> MPPKQTKVVASRKTVMPISRAGRAQIRRKDSNTQNNMNDQGMEDEEIDQQREGMKNQYEQLTAQELNEDMPSKMLEPKNPQAPKNITVYDYYTRKFKTDELVDQMIVHFSMDGDYIWKESNEYKTQEEIRDTKKALIKEAMRKQESEEPGANHDEEAIKQTLRNKFNYNTRECQTINPSIRERGVSTEPPPSDTICGNITQWEIFDAYYAEIMKDHQIENKKKKEVDQDKKQDQSMYSTSFKRCCKIMERMVVQNDQEDKYHDYRYYWSQGDNLEAGKNEGHLLPIWRFSNEKQRKKNVTSICWNPLYPDLFAVSLGSYDFTKQRMGLICLYSLKNTTHPEYAFNCEAGVMCLDFHPKSAALLAVGLYDGTVLVYDIRNKHKKPIYQSTVRNQKHTDPVWQVKWNPDTSKNYNFYSISSDGRVMNWILMKNKLEPEEVILLRLVGKNEEESTLIGLACGLCFDFNKFEPHIFLVGTEEGKIHKCSRAYSGQYQETYNGHLLAVYKVKWNNFHPRTFISASADWTVRIWDSKYTSQIICFDLSMMVVDAVWAPYSSTVFACATMDKVQVYDLNVDK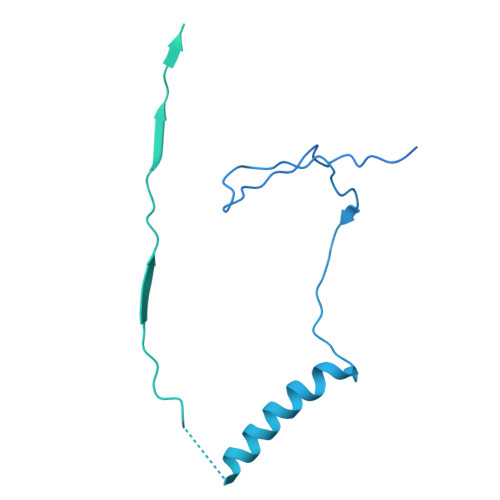LNKLAEQKIVKQPKLTNLSFNYKDPILLVGDSHGGVTLVKLSPNLCKSGPEIKQTEDKKAMEEFKNVKIEDYEREKMENLLAVVSKWEREDA> MIRAVFFDSLGTLNSVEGAAKSHLKIMEEVLGDYPLNPKTLLDEYEKLTREAFSNYAGKPYRPLRDILEEVMRKLAEKYGFKYPENFWEISLRMSQRYGELYPEVVEVLKSLKGKYHVGMITDSDTEQAMAFLDAL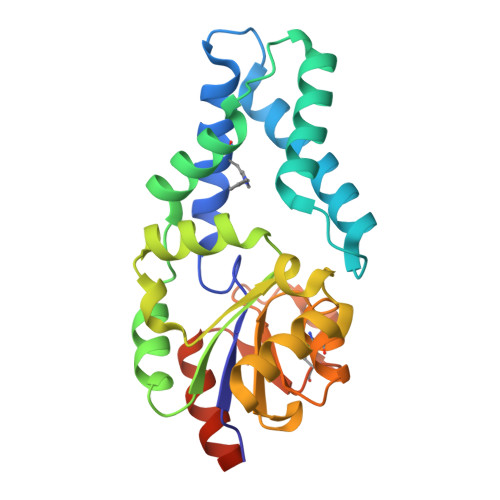GIKDLFDSITTSEEAGFFKPHPRIFELALKKAGVKGEEAVYVGDNPVKDCGGSKNLGMTSILLDRKGEKREFWDKCDFIVSDLREVIKIVDELNGQGSLEHHHHHH6-(4-methylpiperazin-1-yl)-N-[(1R,3S)-5-oxidanyl-2-adamantyl]-2-propylsulfanyl-pyridine-3-carboxamide 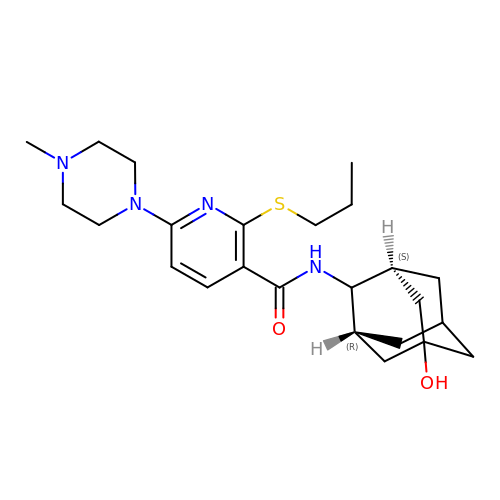| C24 H36 N4 O2 S | HCCPSOBZLRHGQN-OREAVBJWSA-N> MMHRTAARLRMPRKPTPYVRKFLEGCPLPETLVDDIAGANLKSMAPFFTTAPRYIVAAESRLSKLFFHHALYPAGGARRPCRVLIVRGGRSVREPSFTINTGGGRGEVGGGSRGYRDPARRA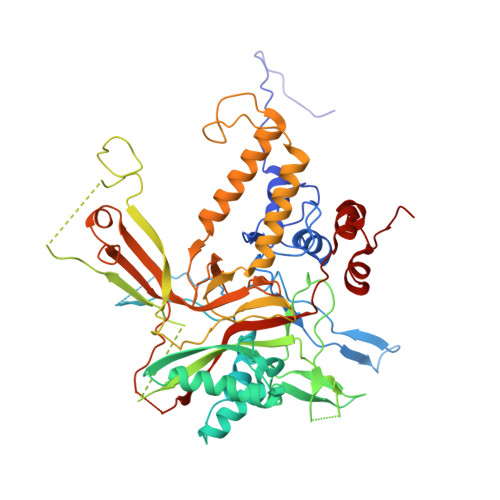YFYARPSTVGPFYSGNGGVSSNVAKCHSGVGSEGAGLVKRASVDGLLSPLCGVIEAHFAVGGTCNDAVATEGDGTESLTKGGEKLCVTLAGLLSGGHGGLMMDDGNCASNVRAAKRVARLLHDAAHHLSSFFYVHTQLPDSALFVSRPEASIASDGKGDGLLPSHLAREKDNDGRPSVEGVAVFRLAGGLEPTVHFAVGAPLSVLQRGVDGTASRGEKNSAEEGLNSAASTTVLPFGHIQCLLRVRTRGGKHCAAGKEGSEGTSNTPWCNTAGNDDITSNFAASGPQIAGGIVEPWKLGVSLDPKVPFFMRTLTEKRPSFSCGEGYLGTCSRSGDVDGNTVNDVSSSSGGSRTRAPGEVHMNHLLVRNDCETYLLPQRELLLSFHVPEEAEAMCKEQNEERMRRQAALGYGSPSHVFAEGPRTFARVLHGMKANLAAVEEASSTFRQGAAEGISPQVNGGSTTSGSSRVYEVRALPGDVVFVPRGWKYSVERIVGTAIIDAVAASTASPREALRAVFRTAPDPPLPQDVVRCDEGHAGAGEMPGGDSSNAEIVGVEVDAFVLCYKPYPVLSNAQASTYVAANYVHSGIDDFYAKGGNDVYHKYT>VGGHEKVISLGFDASKGFHTYAFDWQPGYIKWYVDGVLKHTATANIPSTPGKIMMNLWNGTGVDDWLGSYNGANPLYAEYDWVKYTSNQTGGSFFEPFNSYNSGTWEKADGYSNGGVFNCTWRANNVNFT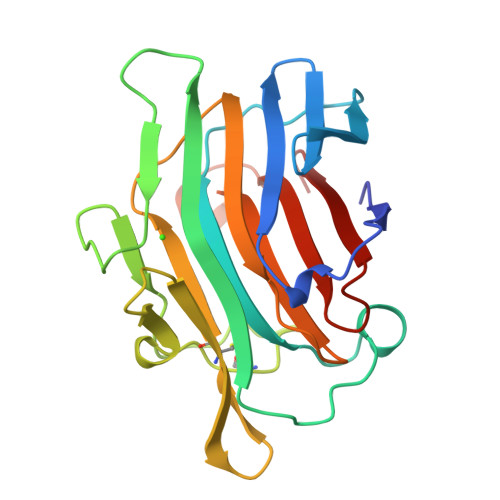NDGKLKLGLTSSAYNKFDCAEYRSTNIYGYGLYEVSMKPAKNTGIVSSFFTYTGPAHGTQWDEIDIEFLGKDTTKVQFNYYTNG[2x]3H-INDOLE-5,6-DIOL | C8 H7 N O2 | 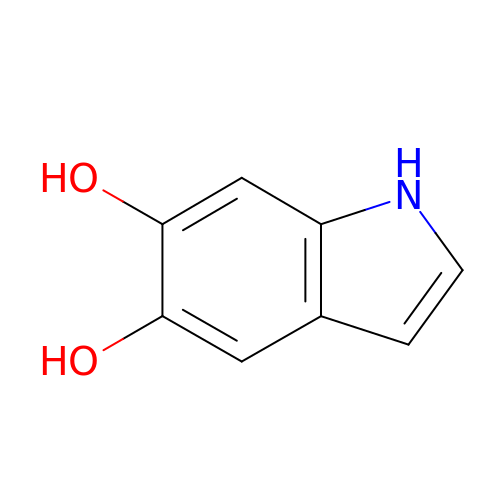SGNZYJXNUURYCH-UHFFFAOYSA-N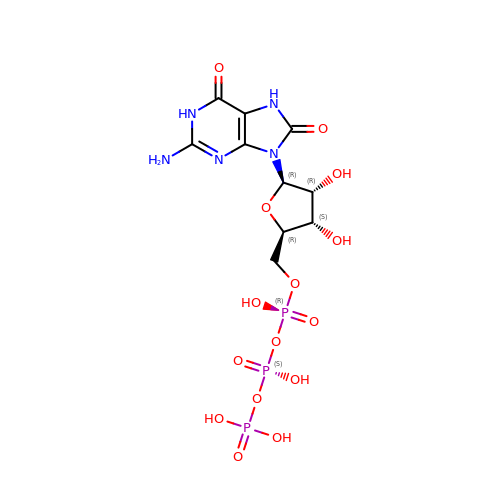8-OXO-GUANOSINE-5'-TRIPHOSPHATE | C10 H16 N5 O15 P3 | JCHLKIQZUXYLPW-UMMCILCDSA-N>[2x]SNHLVKGRSVYELDCIPLWGTVSIQGNRSEMEDAFAVSPHFLKLPIKMLMGDHEGMSPSLTHLTGHFFGVYDGHGGHKVADYCRDRLHFALAEEIERIKDELSKRNTGEGRQVQWDKVFTSCFLTVDGEIEGKIGRAVVGSSDKVLEAVASETVGSTAVVALVCSSHIVVSNCGDSRAVLFRGKEAMPLSVDHKPDREDEYARIENAGGK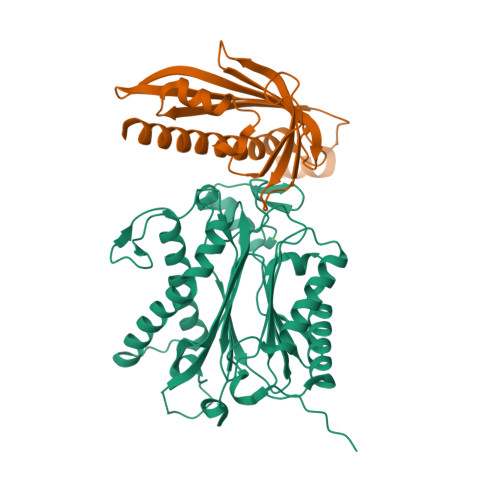VIQWQGARVFGVLAMSRSIGDRYLKPYVIPEPEVTFMPRSREDECLILASDGLWDVMNNQEVCEIARRRILMWHKKNGAPPLAERGKGIDPACQAAADYLSMLALQKGSKDNISIIVIDLKAQRKFKTRT;>[2x]MNGDETKKVESEYIKKHHRHELVESQCSSTLVKHIKAPLHLVWSIVRRFDEPQKYKPFISRCVVQGKKLEVGSVREVDLKSGLPATKSTEVLEILDDNEHILGIRIVGGDHRLKNYSSTISLHSETIDGKTGTLAIESFVVDVPEGNTKEETCFFVEALIQSNLNSLADVTERLQAESMEKKI>WSHPQFEKENLYFQSMANVIKARPKLYVMDNGRMRMDKNWMIAMHNPATIHNPNAQTEFVEFPIYTVLIDHPEGKILFDTSCNPNSMGPQGRWAESTQQMFPWTATEECYLHNRLEQLKVRPEDIRYVVASHLHLNHAGCLEMFTNATIIVHEDEFNGALQCYARNQKEGAYIWADIDAWIKNNLQWRTVKRHEDNILLAEGVKVLNFGSGHAWGMLGLHVELPETGGIILASDAIYTAESYGPPIKPPGIIYDSLGYMNTVERIRRIAQETKSQVWFGHDAEQFKKFRKSTEGYYE[3x]

MLLs degrade N-acyl-L-homoserine lactones (AHLs), molecules that are used in a microbial communication system called quorum sensing (QS) to coordinate a variety of behaviors, including virulence and biofilm formation. We provide the structural and biochemical analysis of the lactonase GcL (WP_017434252.1), isolated from the thermophilic bacteria Parageobacillus caldoxylosilyticus. GcL is a thermostable, highly proficient lactonase with broad substrate specificity (kcat/KM values range between 104 to 106 M–1 s–1) for substrates such as N-butyryl (C4) L-homoserine lactone (HSL) and N-decanoyl (C10)-HSL. The binuclear center, common to all MLLs, is coordinated by five histidine residues and two aspartic acid residues.

Asp122 is also conserved and is involved in coordinating the metal cation. To investigate the importance of these residues, we therefore substituted Tyr223 with phenylalanine and Asp122 with asparagine in GcL, eliminating their role in acid catalysis, and kinetically characterized the resulting GcL variants. The alterations in GcL activity may still suggest that this residue is important, but the interpretation of this effect is complicated by the clear role of this residue in metal coordination. This could be seen through crystallization, where multiple conformations were captured: one where both metals are present at high occupancy, exhibiting an active site configuration very similar to that of the wild-type enzyme; and a second form where the active site shows no bound β-metal (or bound with very low occupancy). In the case of the Asp122Asn variant, the Asp mechanism is no longer accessible due to the mutation of Asp122, leaving only the terminal hydroxide or concerted mechanisms as potential options. Curiously, in this variant, the activation free energy for the terminal hydroxide mechanism increases substantially, leaving the concerted mechanism as the only energetically plausible pathway with calculated activation free energies within 3 kcal mol–1 of the experimental data. Visual examination of our EVB trajectories indicates that during our simulations, the substituted N122 side chain interacts with and stabilizes the terminal hydroxide ion at the Michaelis complex, contributing to higher calculated activation free energies through reactant state stabilization.>[6x]GAMVMRLGDAAELCYNLTSSYLQIAAESDSIIAQTQRAINTTKSILINETFPKWSPLNGEISFSYNGGKDCQVLLLLYLSCLWEYYIVKLSQSQFDGKFHRFPLTKLPTVFIDHDDTFKTLENFIEETSLRYSLSLYESDRDKCETMAEAFETFLQVFPETKAIVI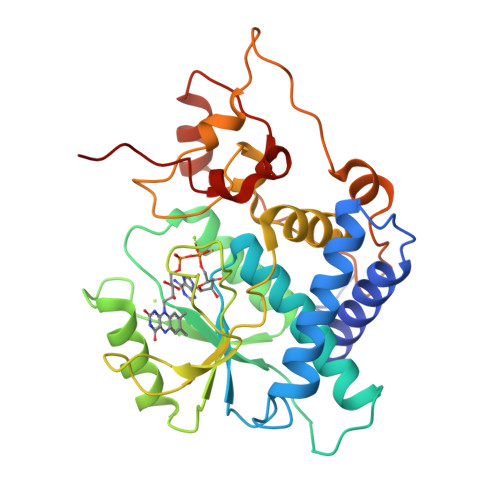GIRHTDPFGEHLKPIQKTDANWPDFYRLQPLLHWNLANIWSFLLYSNEPICELYRYGFTSLGNVEETLPNPHLRKDKNSTPLKLNFEWEIENRYKHNEVTKAEPIPIADEDLVKIENLHEDYYPGWYLVDDKLERAGRIKKK>[2x]GPLGSAPVRSLNCTLRDSQQKSLVMSGPYELKALHLQGQDMEQQVVFSMSFVQGEESNDKIPVALGLKEKNLYLSCVLKDDKPTLQL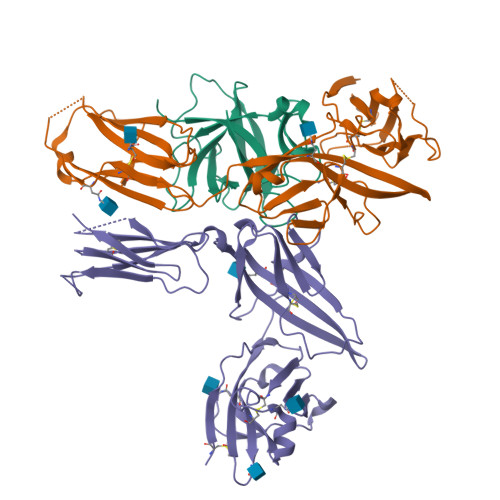ESVDPKNYPKKKMEKRFVFNKIEINNKLEFESAQFPNWYISTSQAENMPVFLGGTKGGQDITDFTMQFVSS;>[2x]EPLEADKCKEREEKIILVSSANEIDVRPCPLNPNEHKGTITWYKDDSKTPVSTEQASRIHQHKEKLWFVPAKVEDSGHYYCVVRNSSYCLRIKISAKFVENEPNLCYNAQAIFKQKLPVAGDGGLVCPYMEFFKNENNELPKLQWYKDCKPLLLDNIHFSGVKDRLIVMNVAEKHRGNYTCHASYTYLGKQYPITRVIEFITLEENKPTRPVIVSPANETMEVDLGSQIQLICNVTGQLSDIAYWKWNGSVIDEDDPVLGEDYYSVENPANKRRSTLITVLNISEIESRFYKHPFTCFAKNTHGIDAAYIQLIYPVTNFQK;>[2x]EPSERCDDWGLDTMRQIQVFEDEPARIKCPLFEHFLKFNYSTAHSAGLTLIWYWTRQDRDLEEPINFRLPENRISKEKDVLWFRPTLLNDTGNYTCMLRNTTYCSKVAFPLEVVQKDSCFNSPMKLPVHKLYIEYGIQRITCPNVDGYFPSSVKPTITWYMGCYKIQNFNNVIPEGMNLSFLIALISNNGNYTCVVTYPENGRTFHLTRTLTVKVVGSPKNAVPPVIHSPNDHVVYEKEPGEELLIPCTVYFSFLMDSRNEVWWTIDGKKPDDITIDVTINESISHSRTEDETRTQILSIKKVTSEDLKRSYVCHARSAKGEVAKAAKVKQKVPAPRYTVELACGFGAT>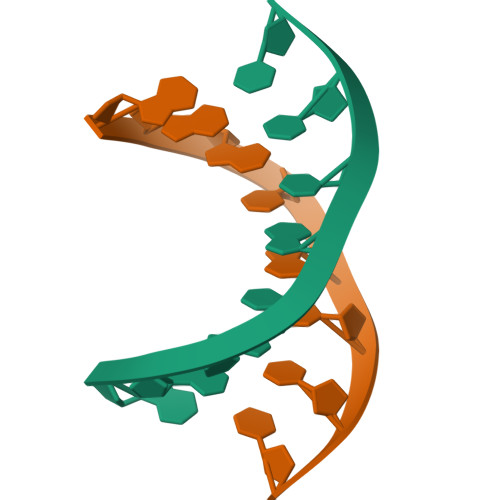 GGGCGCCC> MH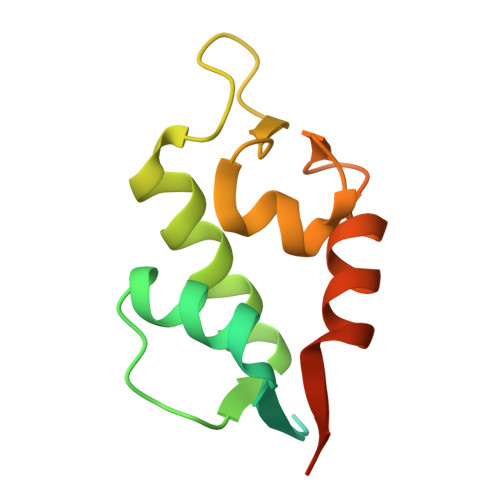HHHHHDDDDKRTTSFSTSAQCSTSDSACRILPGEGTQVHPRAPLLQILKVAGAQEEVFTVKEVMHYLGQYIMMKQLYDKQRQHIVHCHDDPLGELLEVGSFSVKNPSPLYEMLKRNLVILATATTDAAQ General control non-repressible 5 (GCN5)-related N-acetyltransferases (GNATs) are a large superfamily of enzymes, playing prominent roles across a large number of biological processes including aminoglycoside antibiotic resistance, transcription regulation, protein acetylation and stress reaction. The transfer of an acetyl group from acetyl-CoA (AcCoA) to substrates such as aminoglycoside antibiotics alter the fundamental characteristics of these molecules and can render them inactive. Functional GNAT proteins generally contain six (or sometimes seven) β-strands and four α-helices arranged in a (β0)-β1-α1-α2-β2-β3-β4-α3-β5-α4-β6 topology. Here, we describe the structure of a GNAT family member from E. anophelis.

The protein was structured as an α/β protein and comprised of six α-helices and nine β-strands with a topology of β1-α1-α2-β2-β3-β4-α3-α4-β5-α5-β6-α6-β7-β8-β9. The structure exhibits two β-sheets comprised of β-strands 1-4, and β-strands 5, 6, and 9, splayed to create a V-shape. Our structure contained a well-ordered acetyl-CoA molecule bound in the active site. The interface between acetyl-CoA buries 593 Å2 of surface area and mediated by 10 hydrogen bonds. Key residues involved in these hydrogen bond interactions include Ile68, Val70, Asn76, Gly78, Gly80, Gly81, Gln110, Tyr112, and Lys116, and specific interactions are summarized in Table 2. Based on the position of the acetyl-CoA in the structure and well characterized kinetic studies of GNAT enzymes, the most likely active residues are Ser107 and Try114. Approximately 62% of GNATs have been reported to contain a conserved Tyr as a general acid to initiate the catalysis, and the positioning of Tyr114 from our structural analysis is consistent with this. GNATs adopt a wide variety of assemblies, ranging from monomers, dimers, trimers, tetramers, hexamers, and dodecameric (double ring) structures. Analysis of the interfaces present in the crystal using PISA45 suggests the protein is most likely to be a dimer. In this assembly configuration, the two monomers bury a surface area of 1464 Å, and mediated by ten hydrogen bonds and eight salt bridges.

> MAHHHHHHMKDNITIHPHTAGTPIPYDLLLLADPSKELIDQYLTSGELYLAKYNNEIIGCYVLYPWDFETTEIKNIAVAEKFQNQGIGGQLLKDVILKAKNKFYKKLVIGTGNSSTGQLYLYQKYGFRITDIRKNFFKDNYPEPIWENGIECTDMILLTMEL> DYKDDDAMNTSAPPAVSPNITVLAPGKGPWQVAFIGITTGLLSLATVTGNLLVLISFKVNTKLKTVNNYFLLSLACADLIIGTFSMNLYTTYLLMGHWALGTLACDLWLALDYVASNASVMNLLLISFDRYFSVTRPLSYRAKRTPRRAALMIGLAWLVSFVLWAPAILFWQYLVGE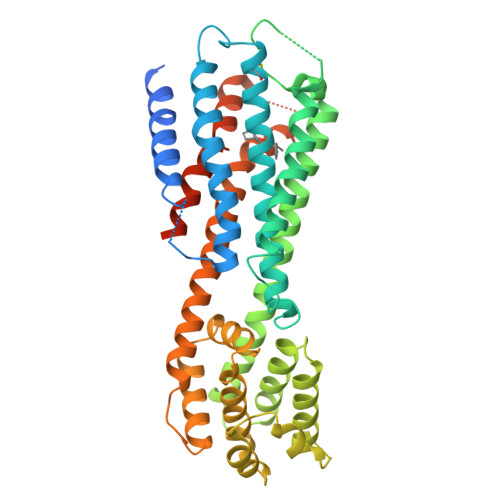RTVLAGQCYIQFLSQPIITFGTAMAAFYLPVTVMCTLYWRIYRFRRRGAEALERAFSLEDDKEALLAALDALAEAFADDAELTALLALLRRLLEDPDLPADELAALRAALTRFPEFREALLALLDRYLATRDLADARDLVWALVLAIASDPRYRPAVAAMIAFGDAEVLRAGLLRGAEALGLPGGEALVEEIMAEAEKEKKAARTLSAILLAFILTWTPYNIMVLVSTFCKDCVPETLWELGYWLCYVNSTININPMCYALCNINPMCYALCNINPMCYALCNHHHHHH>[4x]GPGLKQKIVIKVAMEGNNCRSKAMALVASTGGVDSVALVGDLRDKIEVVGYGIDPIKLISALRKKVGDAELLQVEQAKED;>[2x]METGNKYIEKRAIDLSRERDPNFFDNADI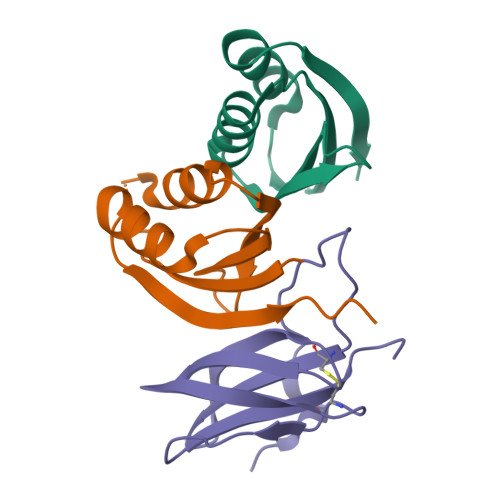PVPECFWFMFKNNVRQDAGTCYSSWKMDKKVGPNWVHIKSDDNCNLSGDFPPGWIVLGKKRPGF> MGLPWELARFSIVKDEVLPHFATNEDLDLANEIISLFKAGKKLGEIDEEIEYLEKIYDHKLVRAFVKLLTRLCEFELDSPIPPIQIRRELFKYGPVLDEKEREDIIQKVSKKLGADIMRFVFSDLDEEKKIIKAPTISAEDLIRWYNLSLLQTLLFKAYKLTVYVSSNWKEIIRRAKWLGLMYFAYDKPLRFEFLGPATLVKLTEKYGRNLAVLLQFI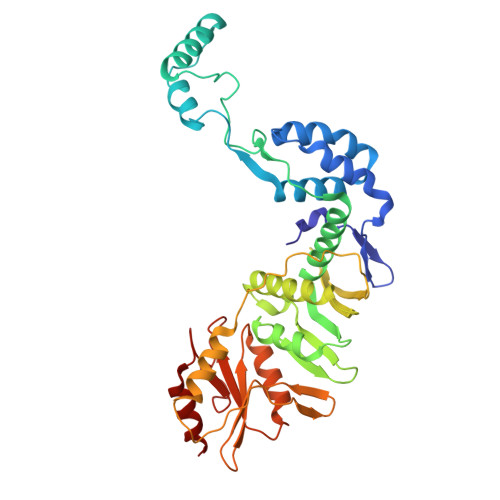ISSQNWKIEAELVLGKKFKRVYKLKLANFKELKELVIDEKRFDSSVEEKFYKDFTNVIKGWKIIREPEPLVVDNRVFIPDFLVEKGNLKVYVEIVGFWTKEYIKEKLDKLKKVKYPILILLNEELGKEKFNGMNVITYKRKIDISLVYKWLRELE>MFLAQEIIRKKRDGHALSDEEIRFFINGIRDNTISEGQIAALAMTIFFHDMTMPERVSLTMAMRDSGTVLDWKSLNLNGPIVDKHSTGGVGDVTSLMLGPMVAACGGYVPMISGRGLGHTGGTLDKLEAIPGFDIFPDDNRFREIIQDVGVAIIGQTSSLAPADKRFYATRDITATVDSIPLITGSILAKKLAEGLDALVMDVKVGSGAFMPTYELSEALAEAIVGVANGAGVRTTALLTDMNQVLASSAGNAVEVREAVQFLTGEYRNPRLFDVTMALCVEMLISGQLAKDDAEARAKLQAVLDNGKAAEVFGRMVAAQKGPSDFVENYDKYLPTAMLSKAVYADTEGFISAM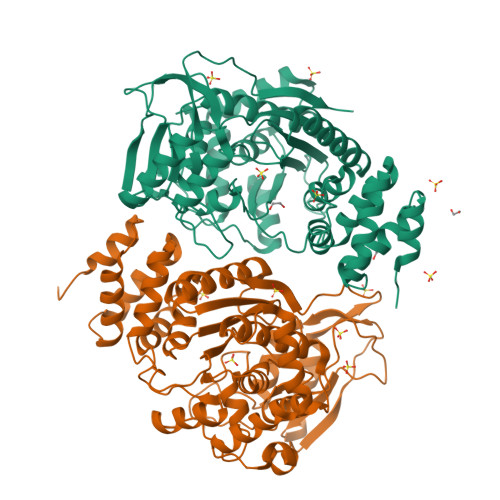DTRALGMAVVSMGGGRRQASDTIDYSVGFTDMARLGDSIDGQRPLAVIHAKDEASWQEAAKAVKAAIILDDKAPASTPSVYRRITE[2x]> MAVTSFLGKAFEKYFYDFSAYEQFGLNRFLSSK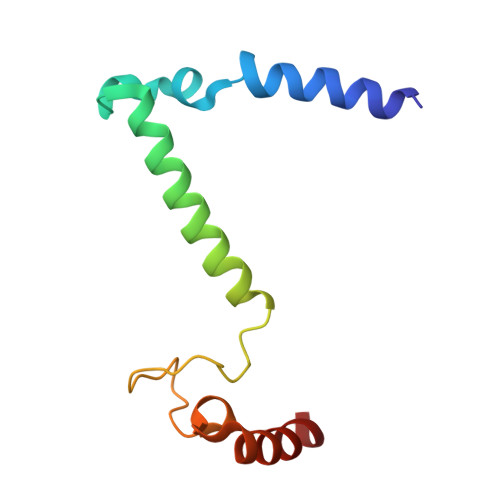GQYVALRHVGFVMVGVNVLLAANFPFNPPFPTIGMCPAGWEGTWVCQADKAKALEMYKEWKKSN>GPGSMKDDHKAQHRFAGLATRAIHSGYRPDPATGAVNAPIYASSTFAQDGVGGLRGGYEYARTGNPTRTALEAALAAVEDAAFGRAFSSGMAAADCALRAMLRPGDHVVIPDDAYGGTFRLIDKVFTG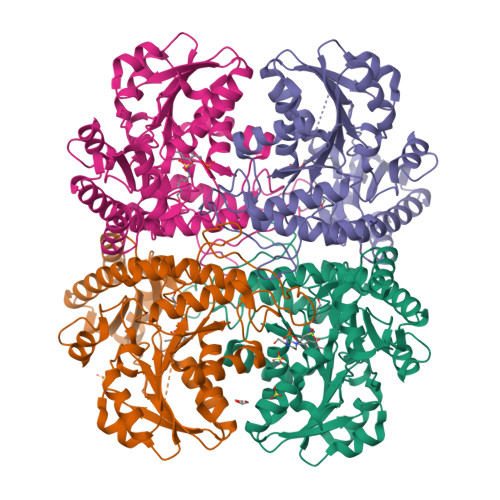WNVEYTPVALADLDAVRAAIRPTTRLIWVETPTNPLLSIADIAGIAQLGADSSAKVLVDNTFASPALQQPLSLGADVVLHSTTKYIGGHSDVVGGALVTNDEELDQSFAFLQNGAGAVPGPFDAYLTMRGLKTLVLRMQRHSENAAAVAEFLAEHPAISTVLYPGLPSHPGHAVAARQMRGFGGMVSVRMRAGRTAAEQLCAKTNIFILAESLGSVESLIEHPSAMTHASTAGSQLEVPDDLVRLSVGIEDVADLLDDLKQALG[4x]beta-D-xylulofuranose 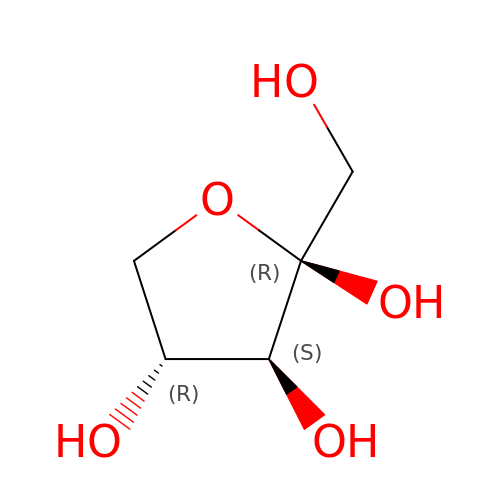| C5 H10 O5 | LQXVFWRQNMEDEE-MROZADKFSA-N> ASFPVEILPFLYLGCAKDSTNLDVLEEFGIKYILNVTPNLPNLFENAGEFKYKQIPISDHWSQNLSQFFPEAISFIDEARGKNCGVLVHSLAGISRSVTVTVAYLMQKL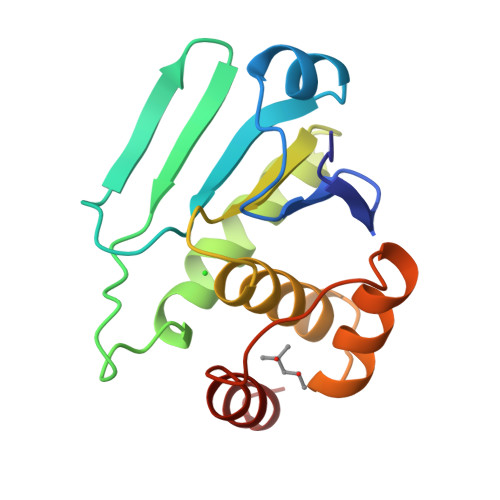NLSMNDAYDIVKMKKSNISPNFNFMGQLLDFERTL>[2x]MGSDKIHHHHHHENLYFQGMANIVFIATSLDGYIADKRGKLDWLHSVPNPNNVDTGFVALMERVDGLVMGRNTLDMVLSFDCDWPYSKP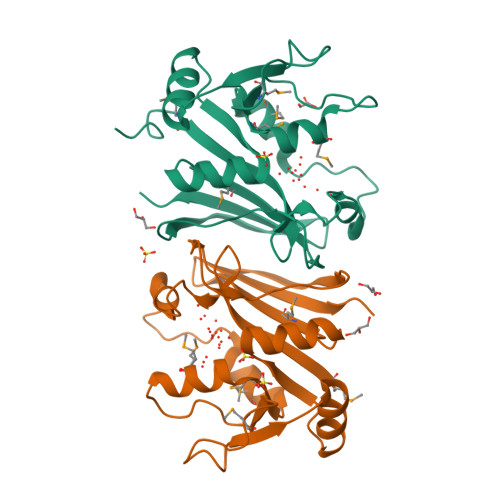VFVLSNTMTEVPQGYEDKVFLVKGKLVDIIADLNAKGFNELYIDGGVTIQNFLKEDLIDEMVITRFPILLGGGVPLFGELESSLSFNVIKSEVVLDSLTQTTYHRKRA> MDRVGKYGLFIKRISPKDADITKESLETVNNMLVFLAEKLTKQANIIIDQKTLRHDAFLWLLTDIQGELGKHSQDFANSVLYGEKELVFP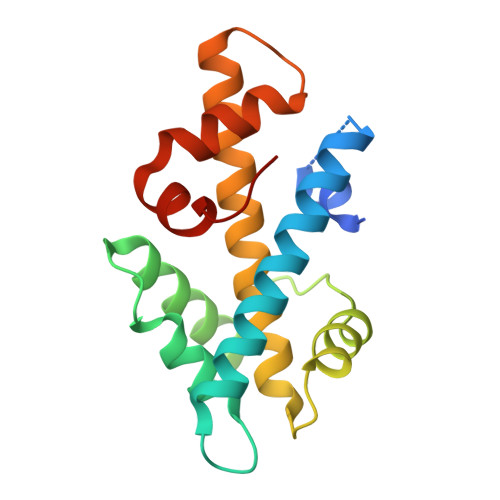TKRTENLMRKNTCLRISQSAVKTLTAILEYFCGQIMEASFSQAKKSKRKRIRPIDIEAAISQDKELHSMFGKGVISGR>MVLPNFKENLEKYAKLLVANGINVQPGHTLALSIDVEQRELAHLIVKEAYALGAHEVIVQWTDDVINREKFLHAPMERLDNVPEYKIAEMNYLLENKASRLGVRSSDPGALNGVDADKLSASAKAMGLAMKPMRIATQSNKVSWTVAAAAGLEWAKKVFPNAASDEEAVDFLWDQIFKTCRVYEADPVKAWEEHAAILKSKADMLNKEQFSALHYTAPGTDLTLGLPKNHVWESAGAVNAQGEEFLPNMPTEEVFTAPDFRRADGYVTSTKPLSYNGNIIEGIKVTFKDGQIVDITAEKGDQVMKDLVFENAGARALGECALVPDPSPISQSGITFFNTLFDENASNHLAIGAAYATSVVDGAEMSEEELEAAGLNRSDVHVDFMIGSNQM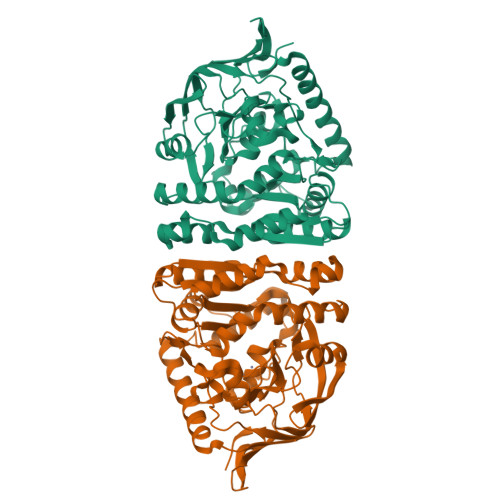DIDGIREDGTRVPLFRNGNWAN[2x]>[2x]MAVLGLQGVRGGVGTTTITAALAWSLQMLGENVLVVDACPDNLLRLSFNVDFTHRQGWARAMLDGQDWRDAGLRYTSQLDLLPFGQLSIEEQENPQHWQTRLSDICSGLQQLKASGRYQWILIDLPRDASQITHQLLSLCDHSLAIVNVDANCHIRLHQQALPDGAHILINNFRIGSQVQDDIYQLWLQSQRRLLPM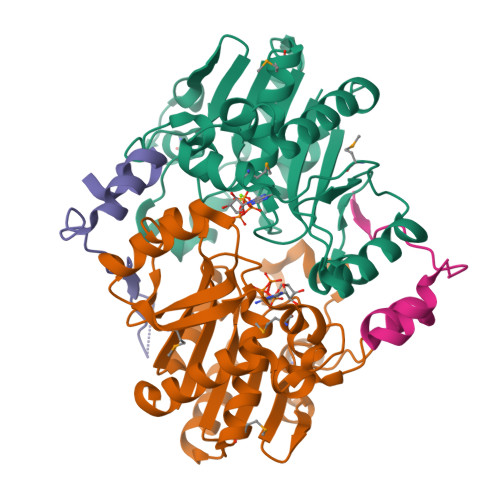LIHRDEAMAECLAAKQPVGEYRSDALAAEEILTLANWCLLNYSGLKTPVGSKSAAALEHHHHHH;>[2x]MNNNEPDTLPDPAIGYIFQNDIVALKQAFSLPDIDYADISQREQLAAALKRWPLLAEFAQQK We report that T. vaginalis has acquired, by lateral gene transfer from bacteria, genes encoding peptidoglycan hydrolases of the NlpC/P60 family. NlpC_A1 and NlpC_A2 consist of the C-terminal NlpC/P60 domain preceded by two bacterial SH3 domains. The NlpC/P60 domain adopts the classical papain-like fold, with a central β-sheet of 5 strands displaying an antiparallel arrangement. Hence, we concluded that NlpC_A1 and NlpC_A2 are dl-endopeptidases with specificity for the tetrapeptides in peptidoglycan and with greater activity toward monomeric muropeptides.

The structures of NlpC_A1 T. vaginalis AG_119910 (TVAG_119910) and NlpC_A2 (TVAG_457240) were determined by X-ray crystallography. Their crystals diffracted to 1.2-Å and 2.3-Å resolution and belonged to the space groups P21221 and P1, respectively. As expected, due to the high sequence identity and similarity (90.2% and 96.4%, respectively), the two structures are essentially identical, with a root mean square deviation (RMSD) value for all atoms of 0.491 Å (1,379 equivalent atoms). A single-residue difference in NlpC_A2 is located near the active site where Leu169 in NlpC_A1 corresponds to Trp169 in NlpC_A2. The tryptophan residue narrows the groove around the active-site cysteine in NlpC_A2. The remaining sequence differences, spread across the protein surface, show no obvious cluster of residues that might influence function. The groove is open and lacks the obvious regulatory elements that are often present in bacterial endogenous peptidases, suggesting that both NlpC_A1 and NlpC_A2 may be unregulated “toxin-like” hydrolases of bacterial PG. Consequently, small-angle X-ray scattering (SAXS) was used to confirm the arrangement of domains within the crystal and that NlpC_A1 and NlpC_A2 are monomeric in solution. The theoretical scattering from the structural models with SAXS curves was consistent with the arrangement of domains present in the crystal, suggesting that the NlpC domain and SH3b domains pack in a concerted arrangement in solution. NlpC_A2 was recently detected from the T. vaginalis secretome.

>[4x]GPGMLSVLLCTSSSYQTQTIGRLTTPGTNLVKAYKTSNPDLNRNCYWLYFDYYVHILGYENGFAHVRIGTEDCWISKDSLEEITIPTKSVTEANIYSEPSRAETIIRYVPANSDVTILDFNCDGFYRINYRGYIGYILEDALQYKWKQVDGANDGERAANLVKTKLGCKYVWAMSGPDTFDCSGLMQWAYNRLDIFMHRTADVQGNHGQLIEDAKDILPGDIITFHTDSEKPTAVTHVGMYVGNGQFIHASTNGYVVRYQDFNSYPYPVSSIRRYWTK2-(6-(((R)-2-amino-2-oxo-1-phenylethyl)carbamoyl)-1-hydroxy-1,3-dihydrobenzo[c][1,2]oxaborol-3-yl)acetic 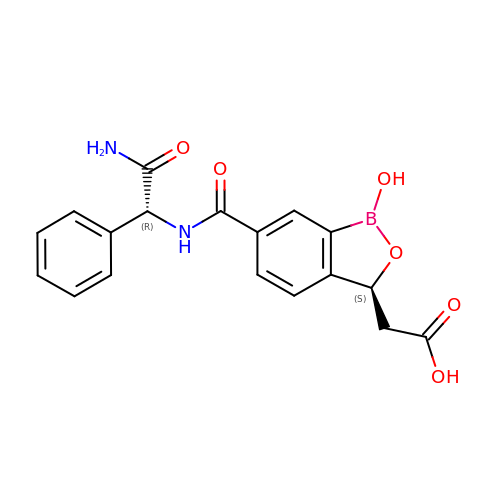acid | C18 H17 B N2 O6 | IKQIDNCBKATNDV-GOEBONIOSA-N The B cell lymphoma 2 (Bcl-2) family of proteins are key regulators of intrinsic apoptosis. The antiapoptotic protein myeloid cell leukemia 1 (Mcl-1), which is associated with high tumor grade, poor survival, and resistance to treatment, has emerged as a promising candidate for treating hematological and solid cancers. The binding interaction is driven by the four hydrophobic residues (L210, L213, V216, and V220 in Mcl-1) in the conserved BH3 domain which bind to four corresponding hydrophobic pockets (P1-4) on the antiapoptotic members. ,− To achieve potent cellular efficacy, Mcl-1 inhibitors require exceptionally low binding affinities (subnanomolar). Herein, we report the structure-guided design of small molecule macrocyclic Mcl-1 inhibitors based on the (R)-methyl-dihydropyrazinoindolone scaffold our group has previously disclosed.

An X-ray cocrystal structure of acyclic inhibitor 8 and Mcl-1 was obtained and is illustrative of the potential benefits of macrocyclization in this series. Two copies of compound 8 bound to Mcl-1 were present in the asymmetric unit, with unambiguous electron density maps of the ligand molecules suggesting two different binding poses of compound 8. The superimposed structures of these two ligand binding poses show a different orientation of the indole 2-carboxylic acid moiety while the other parts of compound 8 remains the same. Figure B,B1 show the favored binding pose, which represents the conformation adopted by the indole 2-carboxylic acid moiety of the ligand in the majority of the cocrystal structures we have obtained in the program. This binding pose provides optimal overlap between the Arg263 residue and the indole ring resulting a cation–π interaction. Additionally, the 2-carboxylic acid moiety forms a polar interaction with the Asn260 side chain (Figure B1). However, as we occasionally observed in our X-ray cocrystals, the ligand may also adopt a binding pose where the indole 2-carboxylic acid is rotated 180° around the C–N amide bond (C1). This binding pose is accompanied by a modest shift in the left-hand portion of the Mcl-1 loop region to accommodate the 2-carboxylic acid moiety, which now forms a hydrogen bonding interaction with the Val258 backbone NH. Inspection of the cocrystal structure of 8 and Mcl-1 shows there is an accessible shelf region that is already partially occupied by the indole 2-carboxylic acid N-substituent (N-ethyl methyl ether in the case of 8) that the tether could occupy (Figure B2).

>[2x]EEDELYRQSLEIISRYLREQATGAKDTKPMGRSGATSRKALETLRRVGDGVQRNHETAFQGMLRKLDIKNEDDVKSLSRVMIHVFSDGVTNWGRIVTLISFGAFVAKHLKTINQESCIEPLAESITDVLVRTKRDWLVKQRGWDGFVEFFHV>MKSLTYFWLFLPVLSTLSLPQDVTRCSAKTNFRRFFSKFNVQAPAVVVLGGYLPIGENQGVNSTWYCAGQHPTASGVHGIFVSHIRGGHGFEIGISQEPFDPSGYQLYLHKATNGNTNATARLRICQFPSIKTLGPTANNDVTIGRNCLFNKAIPAHMSEHSVVGITWDNDRVTVFSDKIYYFYFKNDWSRVATKCYNSGGCAMQYVYEPTYYMLNVTSAGEDGISYQPCTANCIGYAANVFATEPNGHIPEGFSFNNWFLLSNDSTLVHGKVVSNQPLLVNCLLAIPKIYGLGQFFSFNQTIDGVCNGAAVQRAPEALRFNINDTSVILAEGSIVLHTALGTNFSFVCSNSSNPHLATFAIPLG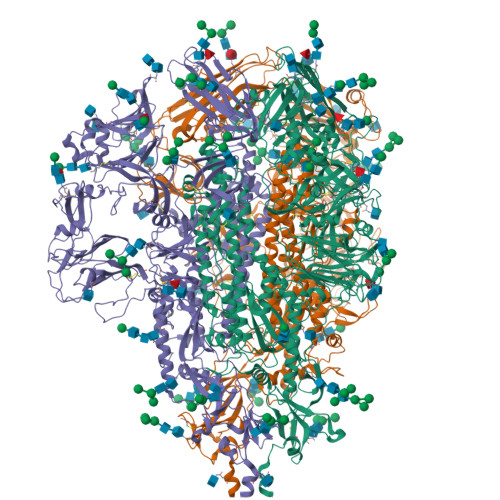ATQVPYYCFFKVDTYNSTVYKFLAVLPPTVREIVITKYGDVYVNGFGYLHLGLLDAVTINFTGHGTDDDVSGFWTIASTNFVDALIEVQGTAIQRILYCDDPVSQLKCSQVAFDLDDGFYPFSSRNLLSHEQPISFVTLPSFNAHSFVNITVSASFGGHSGANLIASDTTINGFSSFCVDTRQFTISLSYNVTNSYGYVSNSQDSNCPFTLQSVNDYLSFSKFCVSTSLLASACTIDLFGYPEFGSGVKFTSLYFQFTKGELITGTPKPLEGVTDVSFMTLDVCTKYTIYGFKGEGIITLTNSSFLAGVYYTSDSGQLLAFKNVTSGAVYSVTPCSFSEQAAYVDDDIVGVISSLSSSTFNSTRELPGFFYHSNDGSNCTEPVLVYSNIGVCKSGSIGYVPSQSGQVKIAPTVTGNISIPTNFSMSIRTEYLQLYNTPVSVDCATYVCNGNSRCKQLLTQYTAACKTIESALQLSARLESVEVNSMLTISEEALQLATISSFNGDGYNFTNVLGVSVYDPARGRVVQKRSFIEDLLFNKVVTNGLGTVDEDYKRCSNGRSVADLVCAQYYSGVMVLPGVVDAEKLHMYSASLIGGMVLGGFTAAAALPFSYAVQARLNYLALQTDVLQRNQQLLAESFNSAIGNITSAFESVKEASSQTSRGLNTVAHALTKVQEVVNSQGAALTQLTVQLQHNFQAISSSIDDIYSRLDILSADVQVDRLITGRLSALNAFVAQTLTKYTEVQASRKLAQQKVNECVKSQSQRYGFCGGDGEHIFSLVQAAPQGLLFLHTVLVPSDFVDVIAIAGLCVNDEIALTLREPGLVLFTHELQNHTATEYFVSSRRMFEPRKPTVSDFVQIESCVVTYVNLTRDQLPDVIPDYIDVNKTRDEILASLPNRTGPSLPLDVFNATYLNLTGEIADLEQRSESLRNTTEELQSLIYNINNTLVDLEWLNRVETYIKWPWWVWLIIFIVLIFVVSLLVFCCISTGFCGCFGCCCACFSGCCRGPRLQPYEVFEKVHVQ[3x]> MARHHHHHHMP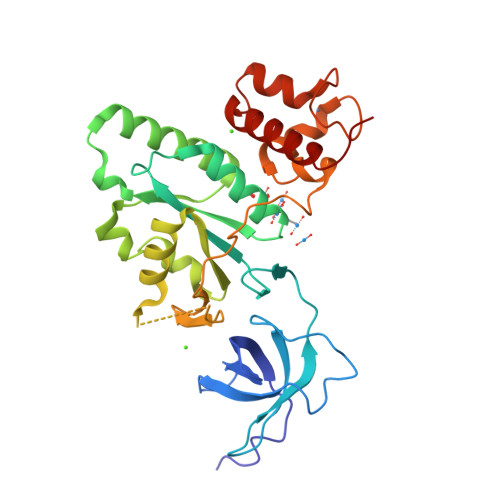EGKIIKALSGFYYVLDESEDSDKVIQCRGRGIFRKNKITPLVGDYVVYQAENDKEGYLMEIKERTNELIRPPICNVDQAVLVFSAVQPSFSTALLDRFLVLVEANDIQPIICITKMDLIEDQDTEDTIQAYAEDYRNIGYDVYLTSSKDQDSLADIIPHFQDKTTVFAGQSGVGKSSLLNAISPELGLRTNEISEHLGRGKHTTRHVELIHTSGGLVADTPGFSSLEFTDIEEEELGYTFPDIREKSSSCKFRGCLHLKEPKCAVKQAVEDGELKQYRYDHYVEFMTEIKDRKPRY>MSTSQEISDPAQATSSAQVKWPRYLEATLGFDNHWHPAAFDHELAEGEFVAVTMLGEKVLLTRAKGEVKAIADGCAHRGVPFSKEPLCFKAGTVSCWYHGWTYDLDDGRLVDVLTSPGSPVIGKIGIKVYPVQVAQGVVFVFIGDEEPHALSEDLPPGFLDEDTHLLGIRRTVQSNWRLGVENGFDTTHIFMHRNSPWVSGNRLAFPYGFVPADRDAMQVYDENWPKGVLDRLSENYMPVFEATLDGETVLSAELTGEEKKVAAQVSVWLPGVLKVDPFPDPTLIQYEFYVPISETQHEYFQVLQ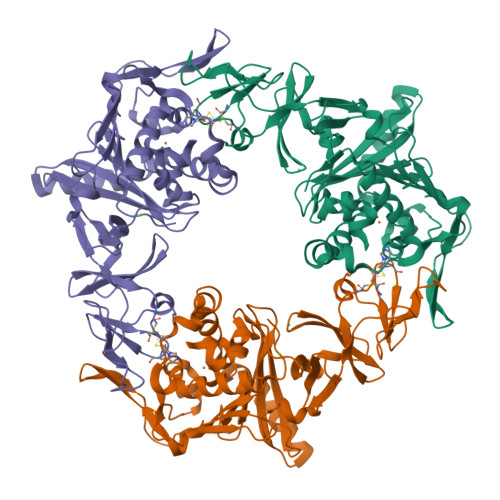RKVEGPEDVKTFEVEFEERWRDDALHGFNDDDVWAREAQQEFYGERDGWSKEQLFPPDMCIVKWRTLASERGRGVRAARVEMSHHHHHH[15x]>SNEKKGTLSIATTHTQARYALPNVISGFIKQYPDVSLHMHQGTPMQIAEMAADGTVDFAIATEALELFGDLIMMPCYRWNRCVIVPHGHPLTKLPKLTLEALAEQPIVTYVFGFTGRSKLDEAFSQRGLVPKVVFTAADADVIKTYVRLGLGVGIVAHMAVDPKLDNDLVILDASHLFESSVTKIGFRRGTFLRGFMCDFIEKFAPHLTRELLAKAVQCHNKAELDE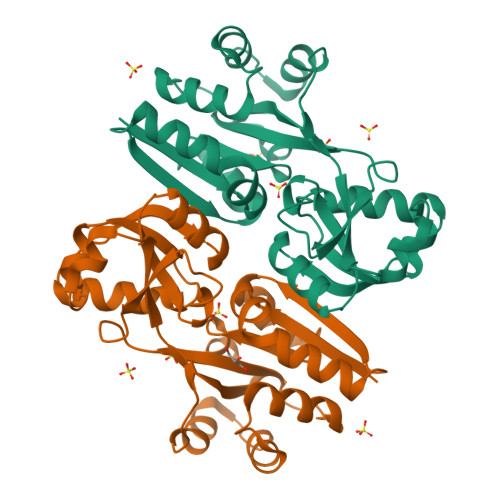LFDGIELPVY[2x]> MTLEKFVDALPIPDTLKPVQQSKEKTYYEVTMEECTHQLHRDLPPTRLWGYNGLFPGPTIEVKRNENVYVKWMNNLPSTHFLPIDHTIHHSDSQHEEPEVKTVVHLHGGVTPDDSDGYPEAWFSKDFE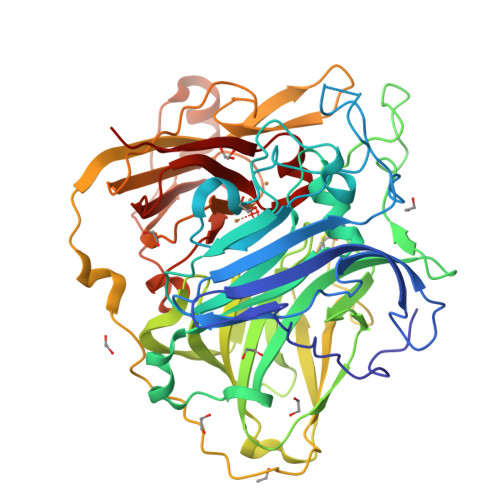QTGPYFKREVYHYPNQQRGAILWYHDHAMALTRLNVYAGLVGAYIIHDPKEKRLKLPSDEYDVPLLITDRTINEDGSLFYPSAPENPSPSLPNPSIVPAFCGETILVNGKVWPYLEVEPRKYRFRVINASNTRTYNLSLDNGGDFIQIGSDGGLLPRSVKLNSFSLAPAERYDIIIDFTAYEGESIILANSAGCGGDVNPETDANIMQFRVTKPLAQKDESRKPKYLASYPSVQHERIQNIRTLKLAGTQDEYGRPVLLLNNKRWHDPVTETPKVGTTEIWSIINPTRGTHPIHLHLVSFRVLDRRPFDIARYQESGELSYTGPAVPPPPSEKGWKDTIQAHAGEVLRIAATFGPYSGRYVWHCHILEHDDYDMMRPMDITDPHK>[2x]SMMELRVGNRYRLGRKIGSGSFGDIYLGTDIAAGEEVAIKLECVKTKHPQLHIESKIYKMMQGGVGIPTIRWCGAEGDYNVMVMELLGPSLEDLFNFCSRKFSLKTVLLLADQMISRIEYIHSKNFIHRDVKPDNFLMGLGKKGNLVYIIDFGLAKKYRDARTHQHIPYRENK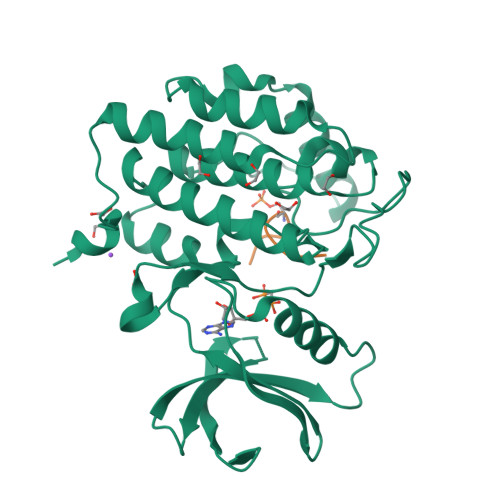NLTGTARYASINTHLGIEQSRRDDLESLGYVLMYFNLGSLPWQGLKAATKRQKYERISEKKMSTPIEVLCKGYPSEFATYLNFCRSLRFDDKPDYSYLRQLFRNLFHRQGFSYDYVFDWNMLK;> RTPSSASTVSVGY> MTNIRVAIVGYGNLGRSVEKLIAKQPDMDLVGIFSRRATLDTKTPVFDVADVDKHADDVDVLFLCMGSATDIPEQAPKF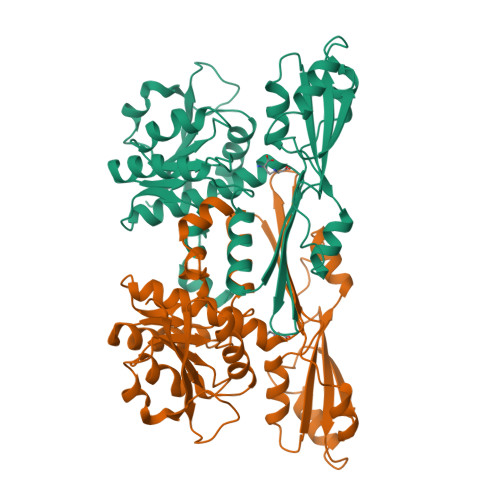AQFACTVDTYDNHRDIPRHRQVMNEAATAAGNVALVSTGWDPGMFSINRVYAAAVLAEHQQHTFWGPGLSQGHSDALRRIPGVQKAVQYTLPSEDALEKARRGEAGDLTGKQTHKRQCFVVADAADHERIENDIRTMPDYFVGYEVEVNFIDEATFDSEHTGMPHGGHVITTGDTGGFNHTVEYILKLDRNPDFTASSQIAFGRAAHRMKQQGQSGAFTVLEVAPYLLSPENLDDLIARDV Rhomboids are evolutionarily conserved serine proteases that cleave transmembrane proteins within the membrane. Rhomboids are a family of intramembrane proteases that use a catalytic dyad of serine and histidine for proteolysis of TM substrates. Here, we describe structures of the Escherichia coli rhomboid GlpG in complex with β-lactam inhibitors. The inhibitors form a single bond to the catalytic serine and the carbonyl oxygen of the inhibitor faces away from the oxyanion hole.

The carbamate substituent is a phenyl (inhibitor L29), isobutyl (inhibitor L61), or a cyclopentyl (inhibitor L62). We have included two data sets of GlpG soaked with L29, which are similar but differ in map quality in certain regions of protein and water molecules. In the first data set, which diffracts to 2.2 Å, loop5 is disordered, while in the second data set, which diffracts to 2.4 Å, the main chain atoms for residues 245–247 of loop5 could be modeled. In the L29 and L62 structures, the carbamate oxygen of the inhibitor hydrogen-bonds to a water molecule, which in turn hydrogen-bonds to the side chain hydroxyl of Y205 and backbone carbonyl of W236. In the L29 structure, the aromatic ring is rotated ∼90° when compared to the L61 and L62 structures. The larger hydrophobic groups such as phenyl (L29), benzyl (L59), or 4-chlorophenyl (L60) inhibited GlpG more potently. In contrast, introduction of smaller and less hydrophobic groups such as a cyclopentane ring or isobutyl group showed a higher half maximal inhibitory concentration (IC50) value. It is evident that the best fit for the S2′ cavity is achieved by larger hydrophobic groups such as an aryl ring (L29), explaining why the smaller isobutyl group is less active. GlpG inhibited with β-lactams L29 or L60 showed 50% recovery of wild-type (WT) activity within 6 and 3.5 hr, respectively. β-lactams with smaller hydrophobic groups, L61 and L62, required >24 hr to attain 50% WT activity. In all structures described here, a water molecule (in the L29 structures) or chloride ion (in the L61 and L62 structures) has been modeled close to the covalently bound inhibitor.

> RAGPVTWVMMIACVVVFIAMQILGDQEVMLWLAWPFDPTLKFEFWRYFTHALMHFSLMHILFNLLWWWYLGGAVEKRLGSGKLIVITLISALLSGYVQQKFSGPWFGGLSGVVYALMGYVWLRGERDPQSGIYLQRGLIIFALIWIVAGWFDLFGMSMANGAHIAGLAVGLAMAFVDSLN> VQFGVMIEKMTGKSALQYNDYGCYCGIGGSHWPVDQTDWCCHAHDCCYGRLEKLGCEPKLEKYLFSVSERGIFCAGRTTCQRLTCECDKRAALCFRRNLGTYNRKYAHYPNKLCTGPTPPC

The mammalian family of secreted phospholipase A2 (sPLA2), which are Ca2+ dependent, low-molecular weight and disulfide-rich enzymes, plays key roles in many physiological functions and pathological processes by catalyzing the hydrolysis of phospholipids at the sn-2 position. GIIE, the closest homolog to GIIA, is regarded as a “hair follicular”, “inflammatory” and “metabolic” sPLA2. The structure of hGIIE consists of a typical set of three major helices (α1, α3 and α4), two β-strands (β1 and β2), and three short helices (α2, α5 and α6) around the second calcium binding site. Similar to hGIIA, hGIIE has seven disulfide bonds.

Two are apo-hGIIE structures at the resolution of 2.0 Å and 1.9 Å, with different crystallization conditions: without (apo-hGIIE_1) or with calcium (apo-hGIIE_2). In the apo-hGIIE_1 structure, crystallized in the condition without calcium, the Ca1 is surprisingly not fully occupied, with only 54% occupancy in this typical calcium binding site. In the apo-hGIIE_1 structure, the occupancy for Ca2 is 57%, which is six-coordinated by the carbonyl oxygen of Asp22, Gly24, Tyr111, carboxyl oxygen of Asp22, amide oxygen of Asn113, and one water molecule. In the apo-hGIIE_1 structure, Ca1 is only 54% occupied and the occupancy for Ca2 is 57%. This raises a possibility that calcium in the second binding site could move to the first calcium binding site when needed. Therefore, hGIIE may have a cost-effective way to use calcium, and Ca2 can act as backup to support the partially occupied Ca1. Similarly in apo-hGIIE structures, a water molecule, part of the second calcium hydration shell, forms a hydrogen bond to the carbonyl oxygen of Cys27 and links the second calcium to the oxyanion.> MGSPKNYIEMKPHPWFFGKIPRAKAEEMLSKQRHDGAFLIRESESAPGD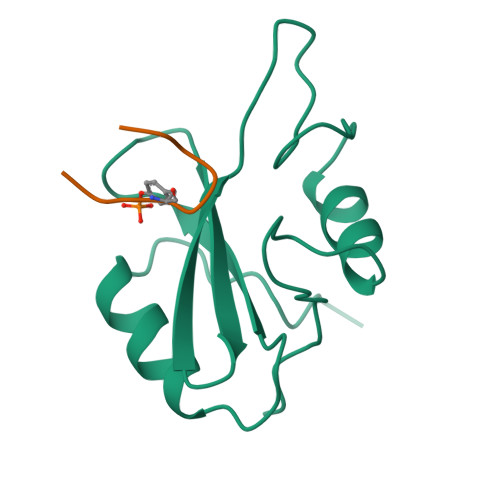FSLSVKFGNDVQHFKVLRDGAGKYFLWVVKFNSLNELVDYHRSTSVSRNQQIFLRDIEQVPQQPTYVQALFDFD;> KPFYVNVEF> MAALGHTLPFYTGTKPTFPMDTTLAVIITIFLTALVTFIIILPGIRGKTRLFWLLRVVTSLFIGAVILAVNFSSEWSVGHVNANTTYKAFSPKWVSVDVGLQIGLGGVNITLTGTP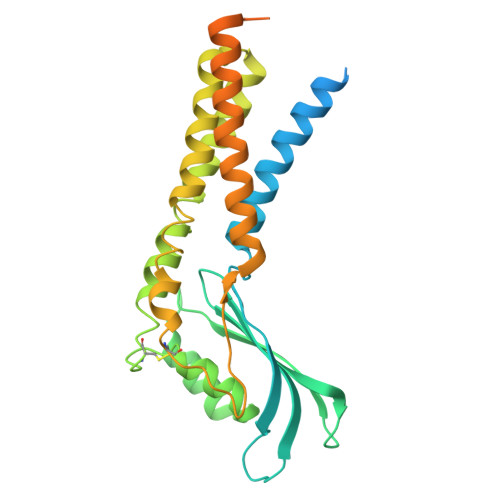VQQLNETINYNEAFAWRLGRSYAEEYAKALEKGLPDPVLYLAEKFTPRSPCGLYNQYRLAGHYASAMLWVAFLCWLLANVMLSMPVLVYGGHMLLATGLFQLLALFFFSMTTSLISPCPLRLGTAVLHTHHGPAFWITLATGLLCILLGLVMAVAHRMQPHRLKAFFNQSSEDPVLEWGSEEGGLLSPHYRSIAESPETQDIPMSVASSETCFKEEHPKESDCSL>[4x]MGHHHHHHGGMITYGSGDLLRADTEALVNTVNCVGVMGKGIALQFKRRYPEMFTAYEKACKRGEVTIGKMFVVDTGQLDGPKHIINFPTKKHWRAPSKLAYIDAGL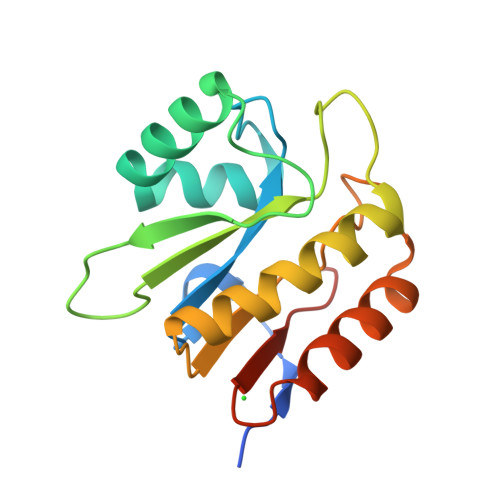IDLIRVIRELNIASVAVPPLGVGNGGLDWEDVEQRLVSAFQQLPDVDAVIYPPSGGSRA> MKHHHHHHPMAIENIYIARHGYRSNWLPKGPYPPPPTGIDNDVPLSEHGVEQAHELANYISKLDVKPEMIFSSPFYRCLETSKPTVEALKIPLYVDRGVGEWYKPDRPIIPEPATHEVMSKFFPSMISPDWEPSIIPSNKGETEEDIFERCHKFWPVFIDRVERKFPNVKTI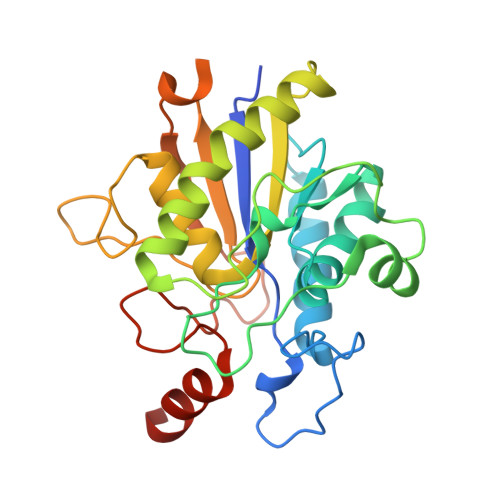MIVTHAATKSALGMNLLKFSSAKEPIDNKGTFIRNGSCAIDKFELVKGENESIPFEEREWKLTMNGNTSFLTNGEEMNWTFMNAFEAGSDADIKARRAAESGKLKME> GSLVREWVGFQQFPAATQEKLIE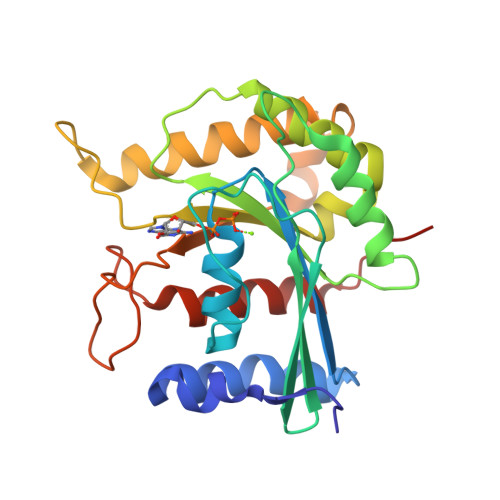FFGKLKQKDMNSMTVLVLGKGGVGKSSTVNSLIGEQVVRVSPFQAEGLRPVMVSRTMGGFTINIIDTPGLVEAGYVNHQALELIKGFLVNRTIDVLLYVDRLDVYAVDELDKQVVIAITQTFGKEIWCKTLLVLTHAQFSPPDELSYETFSSKRSDSLLKTIRAGSKMRKQEFEDSAIAVVYAENSGRCSKNDKDEKALPNGEAWIPNLVKAITDVATNQRKAIHV> MAIASEFSSLPSYAAFATAQEAYEQAVANGDSEVVLKKLKKSLNVAKSEFDRDAAMQRKLEKMADQAMTQMYKQARSEDKRAKVTSAMQTMLFTMLRKLD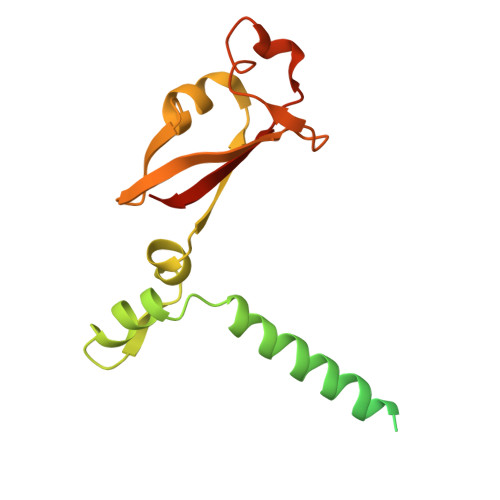NDALNNIINNARDGCVPLNIIPLTTAAKLMVVIPDYNTYKNTCDGTTFTYASALWEIQQVVDADSKIVQLSEISMDNSPNLAWPLIVTALRANSAVKLQ>MADKIKDAKIIFVVGGPGSGKGTQCEKIVAKYGYTHLSSGDLLRAEVASGSERGKQLQAIMQKGELVPLDTVLDMIKDAMIAKADVSKGFLIDGYPREVKQGEEFEKKIGKPCLLLYVDAKAETMVKRLLK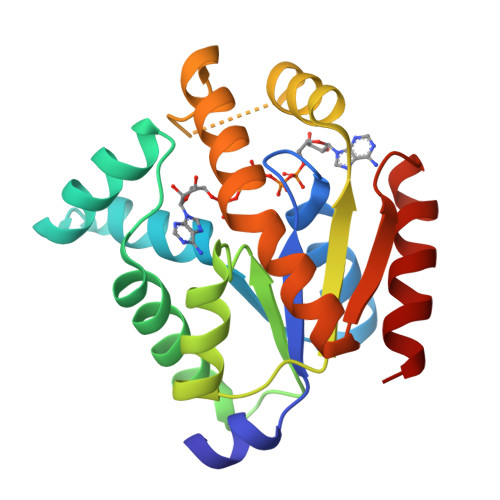RGETSGRSDDNEETIKKRLDLYYKATEPVIAFYEGRGIVKKVDSELAVDDVFAQVSKAIDAL[2x]>MFDFIIDFETMGSGEKAAVIDLAVIAFDPNPEVVETFDELVSRGIKIKFDLKSQKGHRLFTKSTIEWWKNQSPEARKNIAPSDEDVSTIDGIAKFNDYINAHNIDPWKSQGWCRGMSFDFPILVDLIRDIQRLNGVSENELDTFKLEPC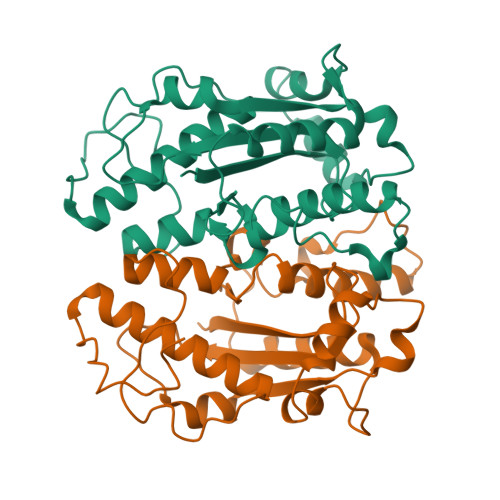KFWNQRDIRTRIEALLLVRDMTTCPLPKGTLDGFVAHDSIHDCAKDILMMKYALRYAMGLEDAPSEEECDPLSLPTKR[4x]> MDQAGIIRDLLIWLEGHLDQPLSLDNVAAKAGYSKWHLQRMFKDVTGHAIGAYIRARRLSKSAVALRLTARPILDIALQYRFDSQQTFTRAFKKQFAQTPALYRRSPEWSAFGIRPPLRLGEFTMPEHKFVTLEDTPLIGVTQSYSCSLEQISDFRHEMRYQFWHDFLGNAPTIPPVLYGLNETRPSQDKDDEQEVFYTTALAQDQADGYVLTGHPVMLQGGEYVMFTYEGLGTGVQEFILTVYGTCMPMLNLTRRKGQDIERYYPAEDA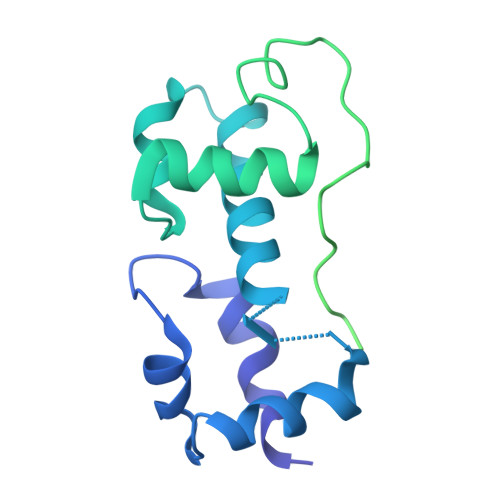KAGDRPINLRCELLIPIRR>HHHHHHGSSQLLPAPLTNDPTAIGPVLPFEELHPRRYPENTATFLTRLRSLPSNHLPQPTLNCLLSAVSDQTKVSEEHLWESLQTILPDSQLSNEETNTLGLSTEHLTALAHLYNFQATVYSDRGPALFGPSDTIKRIDITHTTGPPSHFSPGKRLLGS[2x]

We also reported that the TYMV papain-like cysteine PRO domain involved in the proteolytic processing of the viral replication precursor protein, also displays a DUB activity that was able to rescue the viral polymerase from degradation. The structure of the recombinant TYMV PRO/DUB domain we solved previously (residues 728–879 of the TYMV replication precursor protein) highlighted its homology with members of the ovarian tumor domain-containing (OTU) superfamily of DUBs. In addition, the TYMV PRO/DUB structure displayed a surprisingly exposed and minimal catalytic site, with a Cys783-His869 catalytic dyad instead of the conserved OTU DUB Cys-His-Asp/Asn catalytic triad. The structures reported herein reveal that the loop harboring the 865-GPP-867 motif is a highly mobile flap on the otherwise rigid PRO/DUB framework a result that is confirmed by molecular dynamics simulations.

Given the two similar classes (mild or severe) of DUB activity impairment, whether in loop mutants or distant patch mutants, we also examined the structure of the TYMV PRO/DUB I847A point mutant (hereafter 'I847A'), crystals of which were actually obtained first, and from which we seeded the ΔC5 crystals. The seeding procedure led to the same crystal form, and the I847A crystal is essentially identical to the ΔC5 crystal. The only difference in packing between the ΔC5 and I847A crystals is a slight shift of molecule 'B' with respect to molecule 'A'. Residues 730–877 are ordered in I847A molecule 'A' and residues 732–876 in I847A molecule 'B'. The two I847A molecules appear superimposable to their counterparts in the ΔC5 crystal, with root-mean-square deviation of 0.09 Å for the 143 Cα carbons present and ordered in both 'A' molecules, and 0.23 Å for 141 Cα carbons present and ordered in both 'B' molecules. Importantly, loops 864–868 thus occupy the same positions in the I847A and ΔC5 crystals, i.e. intermediate in 'A' and zipped up in 'B'. The fact that the two mutants I847A and ΔC5 display identical conformations in the same crystal packing environments shows that the mutations themselves have altered neither the overall structure of the molecule, nor the conformation of loop 864–868. Thus, the mobility and zippering of loop 864–868, and the associated changes in the active site conformations as compared to the WT PRO:PRO complex, are properties of the PRO/DUB framework and reflect available conformations of this mobile loop. Additionally, the structure of the I847A mutant confirms that the mutation indeed reduces the hydrophobic surface of the distant patch (black patches in Fig 3). Mutation of these distant patches has allowed the selective disruption of DUB activity in viral PRO/DUB enzymes from EAV, SARS-CoV and MERS-CoV. Such a strategy also proved successful in the case of TYMV PRO/DUB, as we show here that mutants of the distant patch centered on I847 are indeed selectively defective in DUB activity.Macrolide resistance is abundant in pathogenic bacteria, and is most often the result of GTP-dependent macrolide kinases (Mph), ribosomal methyltransferases, or efflux pumps. Mph enzymes inactivate macrolides by phosphorylating the 2′-OH of the essential dimethylamino sugar, preventing it from binding the ribosome, and providing the chemical rationale for the resistance phenotype. Mph enzymes are therefore adaptable resistance enzymes with complex evolutionary paths.

The asymmetric unit of the MphH azithromycin crystal contains two copies of the complex (“complex A” and “complex B”), each showing subtle but important conformational differences. In both complexes, the azithromycin molecule is bound in a deep, electronegative cleft with one face formed by the end of C-terminal domain (i.e., helices α10 and α11), with the other face formed by the apposition of the β hairpin, the highly conserved region of the C-terminal domain containing the catalytic residues, and the nucleotide-positioning loop (NPL; residues 29–33) of the N-terminal domain. However, it was evident that the “complex B” encloses the bound macrolide more intimately and more appropriately for catalysis and this complex dominates our analysis. The position of azithromycin in the macrolide-binding pockets of MphA, MphB, and MphH are similar in that the 2’ rings are oriented appropriately for catalysis, and the macrolactone ring interacts with the β-hairpin regions. However, the azithromycin molecule bound to MphH is positioned ~3 Å closer to the nucleotide binding region as compared to its position in either the MphA or MphB active sites. Consequently, the C3 cladinose ring of azithromycin occupies deeper regions of the binding clefts of MphA or MphB. According to the MphH•azithromycin structure, one of these sites, MphHL31 (MphIM40) interacts with azithromycin; MphHL31 faces toward the desosamine and C6–C7 of the macrolactone ring. MphHA200 (MphIP211) is on the short helix α8 that approaches MphHY198, which forms a key hydrophobic packing interaction with the macrolactone ring close to the methyl on C13 and the ethyl group on C14. MphHW155 (MphIT166) is in α6 that lines the macrolide-binding pocket and lies within 6 Å of the cladinose. In the MphH•azithromycin co-structure, the equivalent MphH positions Leu31 and Ala200 do not interact with the C3 cladinose.

>[2x]QSMPEDLDALLDLAARHGLDLDGGTLRTEEIGLDFRVAFARAHDGGDWVLRLPRRPDVLERAAVEGRLLAMLAPHLDVAVPDWRISTSELIAYPLLPGSPGLTVAADGEVSWHVDMASTVYARSLGSVVAQLHAVDAEAAAATGIEVRSPAQVRGAWRQDLARVGAEFEIAPALRERWEAWLADDGCWPGHSVLTHGELYPAHTLVEDERITAVLDWTTAAVGDPAKDLMFHQVSAPSAIFEVALQAYAEGGGRPWPGLARHCTEMFSAAPLGYGLYALATGEAAHREAAAAALNPPEER N-[5-[(3-methylphenyl)sulfamoyl]-1,3,4-thiadiazol-2-yl]-3-(trifluoromethyloxy)benzamide 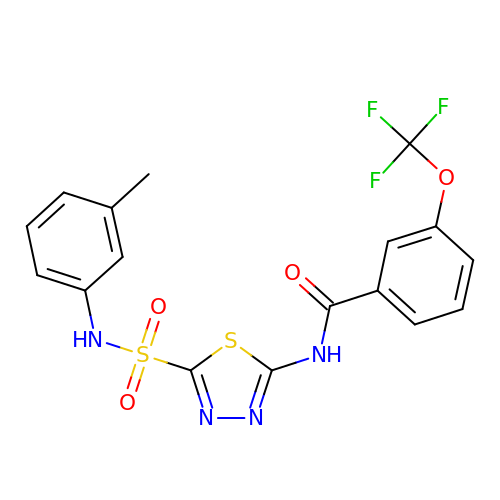| C17 H13 F3 N4 O4 S2 | XHBDIMBSLVRCKA-UHFFFAOYSA-N>MYKDFANFIRTNKKDLLNNWMNEMEKQSDPLINDIAKEPMYEETSIEFVDLIVSNITENGSKFNEKLDDFAEKVVHLGWPIHFVTTGLRVFGLLVYTAMRDEDLFLKREEKPEDDA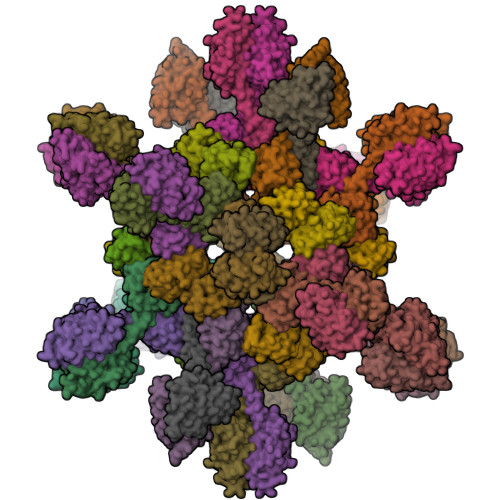YYRFETWLSSMYNKVVTAYADTWEKTVSIQKSALQELSAPLLPIFEKISVMPLIGTIDTERAKLIIENLLIGVVKNRSEVVLIDITGVPVVDTMVAHHIIQASEAVRLVGCQAMLVGIRPEIAQTIVNLGIELDQIITTNTMKKGMERALALTNREIVEKEG[40x];>MGIPILKLGECLLISIQSELDDHTAVEFQEDLLAKIHETSARGVVIDITSIDFIDSFIAKILGDVVSMSKLMGAKVVVTGIQPAVAITLIELGITFSGVLSAMDLESGLEKLKQELGE[20x]>[3x]MGAMIVKEVYE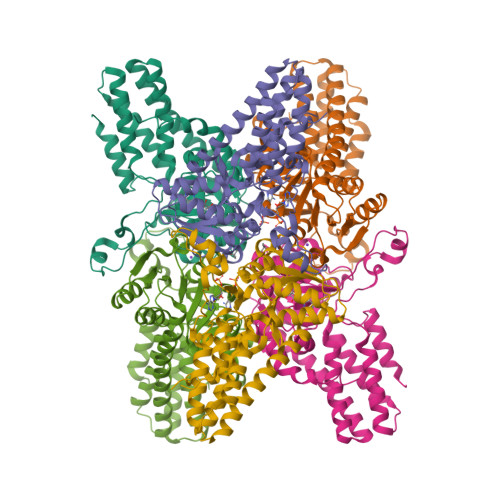TAEKIKSMEIRGAGRIARAAAQALMIQAEKSKAKEPEELWNELKVASKILYNTRPTAVSLPNALRYVMHRVKAAYLGGADLETLRFTAINSAKEFIYNSEKAIERIGEIGAKRIEDGDIIMTHCHSKAAISVMKKAFEQGKNIKVIVTETRPKWQGKITAKELASYGIPVIYIVDSAARHYMKMTDKVVMGADSITANGAVINKIGTSLIALTAKEHRVWVMIAAETYKFHPATMLGQLVEIEMRDPTEVIPEEELRTWPKNIEVWNPAFDVTPPEYIDVIITERGIIPPYAAIDILKEEFGWALKYKEPWED>[2x]AKLTIE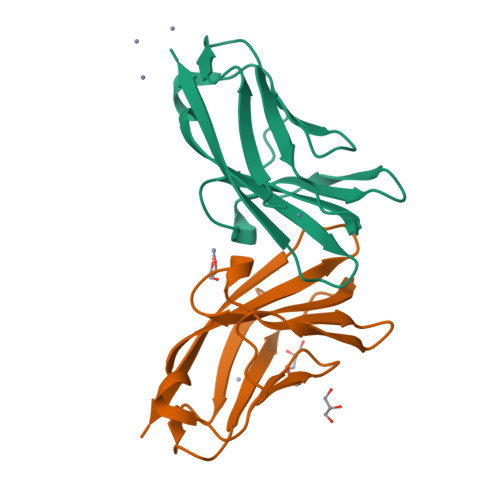STPFNVAEGKEVLLLAHNLPQNRIGYSWYKGERVDGNSLIVGYVIGTQQATPGPAYSGRETIYPNASLLIQNVTQNDTGFYTLQVIKSDLVNEEATGQFHVY> MADELSTMSEPTITNHAQQQAQHLTNTELSSAESKSQDTSQITLKTNREKEQSQDLVSEPTTTELADTDAASMANTGSDATQKSASLPPVNTDVHDWVKTKGAWDKGYKGQGKVVAVIATGIDPAHQSMRISDVSTAKVKSKEDMLARQKAAGINYGSWINDKVVFAHNYVENSDNIKENQFEDFDEDWENFEFDAEAEPKAIKKHKIYRPQSTQAPKETVIKTEETDGSHDIDWTQTDDDTKYESHGMHVTGIVAGNSKEAAATGERFLGIAPEAQVMFMRVFANDIMGSAESLFIKAIEDAVALGADVINLSLGTANGAQLSGSKPLMEAIEKAKKAGVSVVVAAGNERVYGSDHDDPLATNPDYGLVGSPSTGRTPTSVAAINSKWVIQRLMTVKELENRADLNHGKAIYSESVDFKDIKDSLGYDKSHQFAYVKESTDAGYNAQDVKGKIALIERDPNKTYDEMIALAKKHGALGVLIFNNKPGQSNRSMRLTANGMGIPSAFISHEFGKAMSQLNGNGTGSLEFDSVVSKAPSQKGNEMNHFSNWGLTSDGYLKPDITAPGGDIYSTYNDNHYGSQTGTAMASPQIAGASLLVKQYLEKTQPNLPKEKIADIVKNLLMSNAQIHVNPETKTTTSPRQQGAGLLNIDGAVTSGLYVTGKDNYGSISLGNITDTMTFDVTVHNLSNKDKTLRYDTELLTDHVDPQKGRFTLTSHSLKTYQGGEVTVPANGKVTVRVTMDVSQFTKELTKQMPNGYYLEGFVRFRDSQDDQLNRVNIPFVGFKGQFENLAVAEESIYRLKSQGKTGFYFDESGPKDDIYVGKHFTGLVTLGSETNVSTKTISDNGLHTLGTFKNADGKFILEKNAQGNPVLAISPNGDNNQDFAAFKGVFLRKYQGLKASVYHASDKEHKNPLWVSPESFKGDKNFNSDIRFAKSTTLLGTAFSGKSLTGAELPDGHYHYVVSYYPDVVGAKRQEMTFDMILDRQKPVLSQATFDPETNRFKPEPLKDRGLAGVRKDSVFYLERKDNKPYTVTINDSYKYVSVEDNKTFVERQADGSFILPLDKAKLGDFYYMVEDFAGNVAIAKLGDHLPQTLGKTPIKLKLTDGNYQTKETLKDNLEMTQSDTGLVTNQAQLAVVHRNQPQSQLTKMNQDFFISPNEDGNKDFVAFKGLKNNVYNDLTVNVYAKDDHQKQTPIWSSQAGASVSAIESTAWYGITARGSKVMPGDYQYVVTYRDEHGKEHQKQYTISVNDKKPMITQGRFDTINGVDHFTPDKTKALDSSGIVREEVFYLAKKNGRKFDVTEGKDGITVSDNKVYIPKNPDGSYTISKRDGVTLSDYYYLVEDRAGNVSFATLRDLKAVGKDKAVVNFGLDLPVPEDKQIVNFTYLVRDADGKPIENLEYYNNSGNSLILPYGKYTVELLTYDTNAAKLESDKIVSFTLSADNNFQQVTFKITMLATSQITAHFDHLLPEGSRVSLKTAQDQLIPLEQSLYVPKAYGKTVQEGTYEVVVSLPKGYRIEGNTKVNTLPNEVHELSLRLVKVGDASDSTGDHKVMSKNNSQALTASATPTKSTTSATAKALEHHHHHH

The S. pyogenes Cell Envelope Proteinase (SpyCEP) is a highly conserved surface-exposed serine protease that cleaves and inactivates all ELR+ chemokines (containing the N-terminal glutamate leucine arginine motif), notably CXCL8, mediating evasion of immune system clearance strategies and systemic dissemination. SpyCEP is a 180 kDa heterodimer made of two non-covalently linked polypeptides derived from the full-length protein by an intramolecular autocatalytic processing event. The N- and C-terminal fragments are 30 and 150 kDa respectively, and both contribute residues to the catalytic triad (D151 from the N-terminal fragment, H279 and S617 from the C-terminal fragment). Inactivation of the SpyCEP protease activity by amino acid substitution of the residues constituting its catalytic triad should result in a safer single polypeptide vaccine antigen.

Extensive screening using crystals suitable for X-ray diffraction ultimately yielded a novel structure of the full-length ectodomain harbouring the double mutation in the active site, SpyCEP(D151A, S617A), at 2.2 Å resolution, a notable improvement on the resolution of the three previously reported structures. The domain architecture of the SpyCEP(D151A, S617A) mutant matches that observed in the published SpyCEP structures, as expected, with nine distinct folded domains (D1–D9). SpyCEP is significantly larger than the C5a peptidase and has an additional four domains (D6:T1147-K1286; D7:K1287-K1396; D8:D1397-M1489; D9:L1490-A1578) before the linkage to the cell wall. Surprisingly, the two C-terminal domains (D8 and D9) in SpyCEP coil back on the structure and contact the protease domain, an interaction that might retain this distal protease domain proximal to the cell wall. Furthermore, three tightly bound calcium ions present within the interfacial regions of D4–D7 also appear to stabilise the overall architecture of SpyCEP. However, electron density was only observed for residues 116–1574 of the ectodomain (MW ~160 kDa) in all SpyCEP crystal structures, with residues 34–115 and 1575–1613 remaining uncharacterized. Significant structural differences exist between the two double mutants, and these localise to the PA domain and a neighbouring ß-hairpin that supports the relative positions of the PA and protease domains. This region is completely disordered in SpyCEP (H279A, S617A) as native contacts between the catalytic H279 and Q613 at the base of the ß-hairpin are removed by mutation of the histidine to alanine. In light of this, refinement of our SpyCEP structure by using the PA domain and the rest of the protein as separate search models for molecular replacement gave significant improvements in electron density maps over using the whole SpyCEP structure, and a shift in its relative position was observed compared to the published structures. In molecular dynamics the greatest mobility is observed for the PA domain.>[4x]EEGQKVDHCARHGEKLLLFCQEDSKVICWLCERSQEHRGHHTFLMEEVAQEYHVKLQTALEMLRQKQQEAETERNQVAKRVPKAPPEEKEALIARGKALGEQTQYMRELISELEHRLQGSMMDLLQGVDGIIKRIENMTLK

TRIM5α is a restriction factor that intercepts the incoming capsids of diverse retroviruses, including HIV-1, and inhibits viral replication. Like all TRIM proteins, TRIM5α consists of an N-terminal tripartite or RBCC motif (RING, B-box 2, and coiled-coil domains), followed by a C-terminal domain. Higher-order assembly of TRIM5α requires the B-box 2 domain, which is thought to mediate three-fold symmetric interactions that connect coiled-coil mediated TRIM5α dimers into a hexagonal net. We therefore engineered artificial constructs – which we call miniTRIMs – that retain the integrated B-box/coiled-coil fold of the full-length dimer but are more amenable to biochemical and structural analyses.

A P212121 crystal contained two trimers in the asymmetric unit (3.26 Å resolution, R/Rfree = 0.26/0.30), a C2 form contained one dimer (2.1 Å, R/Rfree = 0.18/0.22), and a P1 form contained two dimers (2.3 Å, R/Rfree = 0.22/0.26). The dimer is quasi-equivalent to the trimer: the same sets of residues make the same interactions but with valence of two instead of three. The dimer buries a smaller surface area per subunit (450 Å2) compared to the trimer. Another distinction is that the first two turns of the coiled-coil helix are overwound and bent in the dimer form, which might indicate some structural communication between the interacting B-boxes and the coiled-coil domain. Interestingly, B-box dimerization is associated with local bending of the first two turns of the coiled-coil helix, as well as altered packing of the B-box against the coiled-coil domain. This suggests a potential mechanism of allosteric communication that can link B-box oligomerization and coiled-coil dynamics. In context of the full-length protein, assembly cooperativity drives the B-box into the trimer form, and so the B-box dimer might represent an intermediate state that can incorporate an additional B-box domain to form the trimer. Consistent with this interpretation, our structures indicate that the Bcc miniTRIM dimers can open slightly like a clam shell, which we imagine can lead to a wider opening and provide access to a third subunit. In principle, however, B-box dimers provide a means for extending the TRIM array in regions where the local assembly environment disfavors trimers. The catalytically active RING configuration is more structurally compatible with a B-box dimer, and it is therefore possible that the B-box switches its oligomeric configuration to facilitate enzymatic function.> GPLGSPEFGYWITCCPTCDVDINTWVPFYSTELNKPA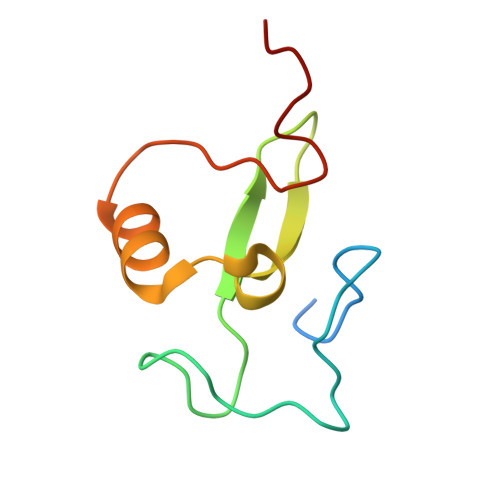MIYCSHGDGHWVHAQCMDLEERTLIHLSEGSNKYYCNEHVQIARA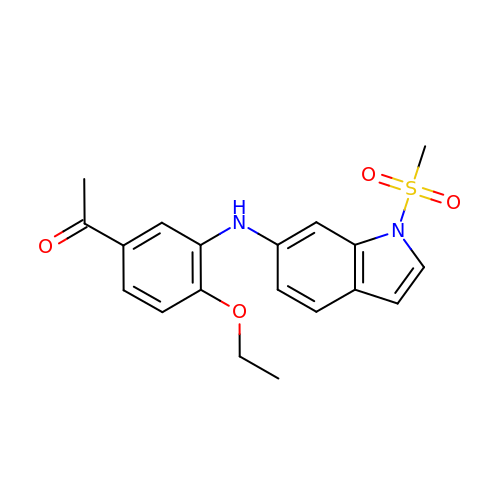1-[4-ethoxy-3-[(1-methylsulfonylindol-6-yl)amino]phenyl]ethanone | C19 H20 N2 O4 S | OCKRWFCZZXKGGR-UHFFFAOYSA-N Naproxen Methyl Ester | C15 H16 O3 | 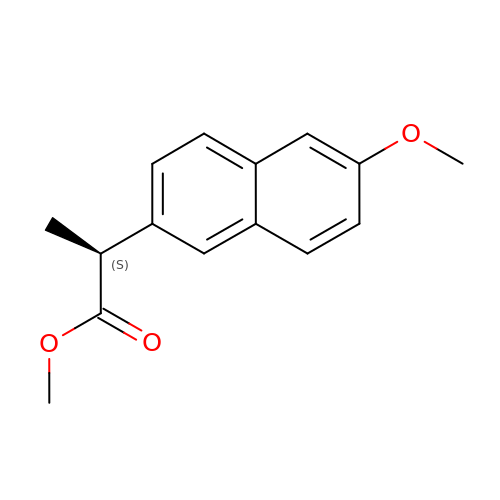ZFYFBPCRUQZGJE-JTQLQIEISA-N> VDCSEYPKPACTLEYRPLCGSDNKTYANKCNFCNAVVESNGTLTLSHF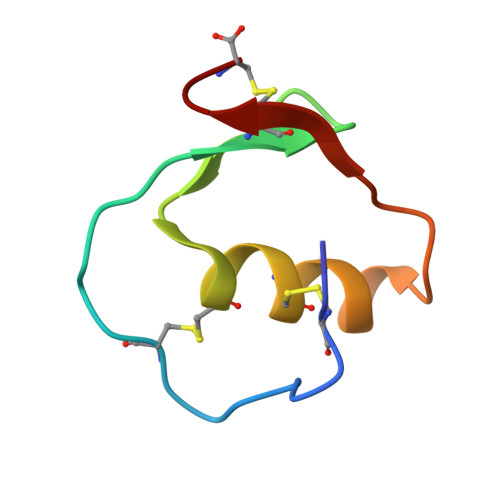GKC> MAAEAETKAMITLRSCEGQVFEVAEAVAMESQTIRHMIEDKCADTGIPLPNVSAKILSKVIEYCSKHVEARGGAA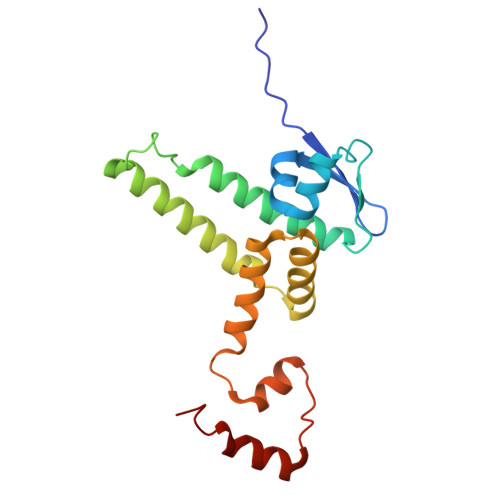AAADGDAPAPAAVEANKAVEDELKTFDAEFVKVDQSTLFDLILAANYLNIKGLLDLTCQTVADMIKGKTPEEIRKTFNIKNDFTPEEEEEVRRENQWAFE> GDELLNICMNAKHHKRVPSPEDKLYEECIPWKDNACCTLTTSWEAHLDVSPLYNFSLFHCGLLMPGCRKHFIQAICFYECSPNLGPWIQPVGSLGWEVAPSGQGERVVNVPLCQEDCEEWWEDCRMSYTCKSNWRGGWDWSQGKNRC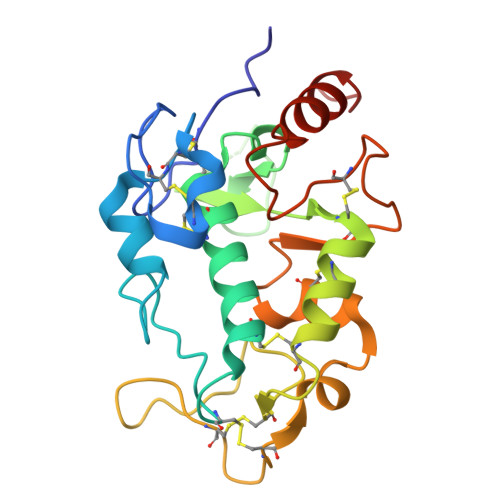PKGAQCLPFSHYFPTPADLCEKTWSNSFKASPERRNSGRCLQKWFEPAQGNPNVAVARLFASGRLVPR> MSKNRSSLQSGPLNSELLEEQKQEIYEAFSLFDMNNDGFLDYHELKVAMKALGFELPKREILDLIDEYDSEGRHLMKY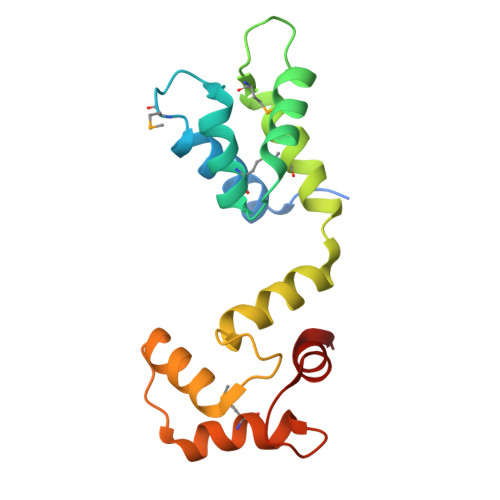DDFYIVMGEKILKRDPLDEIKRAFQLFDDDHTGKISIKNLRRVAKELGETLTDEELRAMIEEFDLDGDGEINENEFIAICTDS> MSQNLFNVEDYRKLAQKRLPKMVYDYLEGGAEDEYGVKHNRDVFQQWRFKPKRLVDVSRRSLQAEVLGKRQSMPLLIGPTGLNGALWPKGDLALARAATKAGIPFVLSTASNMSIEDLARQCDGDLWFQLYVIHREIAQGMVLKALHTGYTTLVLTTDVAVNGYRERDLHNRFKIPPFLTLKNFEGIDLGKMDKANLEMQAALMSRQMDASFNWEALRWLRDLWPHKLLVKGLLSAEDADRCIAEGADGVILSNHGGRQLDCAISPMEVLAQSVAKTGKPVLIDSGFRRGSDIVKALALGAEAVLLGRATLYGLAARGETGVDEVLTLLKADIDRTLAQIGCPDITSLSPDYLQNEGVTNT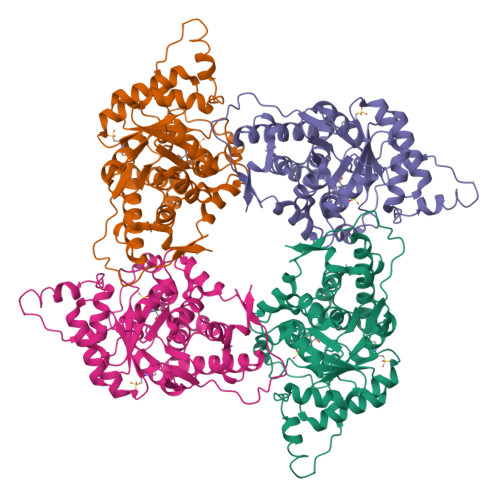APVDHLIGKGTHAHHHHHH>GPAGNKASKQKFCHHCNSRSASAPPGTSTIHYEKSWLYRHCSLQQRDRQAQKSGQLFSGLLALNVVFLGSAFISSMIFNHVAITLADVWILLSILKVLCLCWIIYYLLGTSRQPHAVLYRDTHAAPVWIRGSLLLFGTFSILLNVFQIGYSVIQINCKSKVEIVFPSIEILFVATQAFFLWHHSKDCIQVQHNLTRCGLMLTIATNLLLWLLAVTNDSIHMEIESQLREVEQRLAGNETDSCACPNTTTCKVFQKGYILLYPFNTEYCLICCSVLYVMWKNVGRRISHHHIAHIKPKFKLQGVVFGPLLGAAAVIIGICVFMMYQIQATGSAPNYQVFVLYYSYYIVLLPLMCVVAIIGT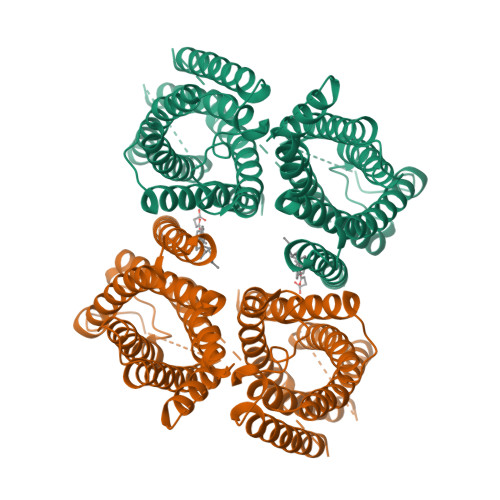IIHTLEKRELDTLKNPTRSLDVVLLMGAALGQIAMSYFSIVAIVATNPRDMLNSLILSYSVLLIFQYITQNIFIIDGLQRQPFAKEEEVSEEHNREAPDQRRVSVLELGQEFRRVSLSYIHTYSHLGWKRKALKEISFFLVLCNIILWIMPTFGAHPVFENGLQKSFYGYSTWFAIVNFGLPLSVFYRMHSVGGLLEVYVSA[2x]>[4x]MAMTLRDMDAVRPVNREAVDRHKARMRDEVRAFRLRELRAAQSLTQVQVAALAHIRQSRVSSIENGDIGSAQVNTLRKYVSALGGELDITVRLGDETFTLA

In the present study, we elucidated the crystal structure of Mycobacterium tuberculosis H37Rv HigA2 (hereafter referred to as MtHigA2), which contains an HTH motif. The HigA antitoxin represses the transcription of HigBA or forms a stable HigBA complex, thereby preventing the ribonuclease activity of the HigB toxin and the associated cytotoxic events. Structural studies of MtHigA2 confirmed that it has three regions: (i) a disordered N-terminus that is liable to cleavage, (ii) an α-helix bundle containing an HTH motif for DNA binding and (iii) a β-lid for dimerization. The antitoxin MtHigA2 has two binding partners: DNA and the toxin MtHigB2.

The crystal structure of MtHigA2 was determined from three distinct crystal forms. Form I belonged to space group P212121 and was determined to 2.0 Å resolution, form II packed in space group P43212 and was determined to 3.2 Å resolution, and form III was solved in space group P3121 to 3.4 Å resolution. However, the N-terminal ∼25 residues are unstructured in all three observed crystal forms. All dimers share the β-lid as their major dimeric interface, but the position of the α-helix bundle varies. When the different dimers are aligned based on a single HTH motif from one monomer, the corresponding motif in the dimer pair shows a different relative position. The flexibility in dimerization leads to drastic changes in the locations of positively charged residues on the HTH motif, including His54, Arg56 and Arg59. To predict the physiological dimer, each form was submitted to the PISA server to calculate the strength of the dimer interface. Interestingly, all of the forms had similarly favourable dissociation energies (ΔG): −14, −15 and −17 kcal mol−1 for forms I, II and III, respectively. This suggests that the flexibility of the β-lid does not impact the formation of a stable dimer and is likely to contribute to function. The three different crystal structures in our study reveal the flexibility in dimerization mode while anchored by the β-lid.>MNTVSPAKKKVIIIGAGIAGLKAASTLHQNGIQDCLVLEARDRVGGRLQTVTGYQGRKYDIGASWHHDTLTNPLFLEEAQLSLNDGRTRFVFDDDNFIYIDEERGRVDHDKELLLEIVDNEMSKFAELEFHQHLGVSDCSFFQLVMKYLLQRRQFLTNDQIRYLPQLCRYLELWHGLDWKLLSAKDTYFGHQGRNAFALNYDSVVQRIAQSFPQNWLKLSCEVKSITREPSKNVTVNCEDGTVYN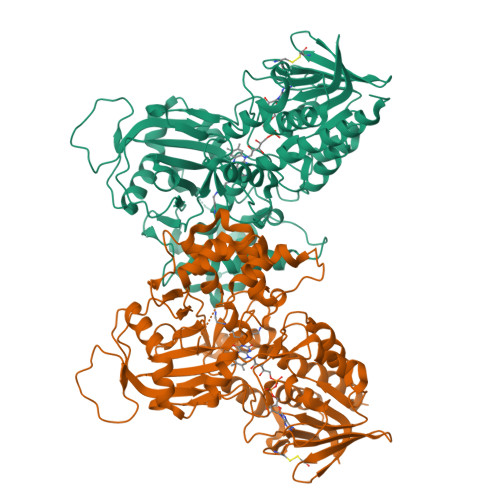ADYVIITVPQSVLNLSVQPEKNLRGRIEFQPPLKPVIQDAFDKIHFGALGKVIFEFEECCWSNESSKIVTLANSTNEFVEIVRNAENLDELDSMLEREDSQKHTSVTCWSQPLFFVNLSKSTGVASFMMLMQAPLTNHIESIREDKERLFSFFQPVLNKIMKCLDSEDVIDGMRPIENIANANKPVLRNIIVSNWTRDPYSRGAYSACFPGDDPVDMVVAMSNGQDSRIRFAGEHTIMDGAGCAYGAWESGRREATRISDLLKLEHHH[4x]> MSEYMDDVDREFINCLFPSYLLQQPVAYDLWILYLQHRKLFHKLKNTNLINADENPTGVGMGRTKLTALTRKEIWSKLMNLGVLGTISFEAVNDDYLIQVYKYFYPDVNDFTLRFGVKDSNKNSVRVMKASSDMRKNAQELLEPVLSEREMALNSNTSLENDRNDDDDDDDDDDDDDDDDDDDDDESDLESLEGEVDTDTDDNNEGDGSDNHEEGGEEGSRGADADVSSAQQRAERVADPWIYQRSRSAINIETESRNLWDTSDKNSGLQYYPPDQSPSSSFSSPRVSSGNDKNDNEATNVLSNSGSKKKNSMIPDIYKILGYFLPSRWQAQPNNSLQLSQDGITHLQPNPDYHSYMTYERSSASSASTRNRLRTSFENSGKVDFAVTWANKSLPDNKLTIFYYEIKVLSVTSTESAENSNIVIGYKLVENELMEATTKKSVSRSSVAGSSSSLGGSNNMSSNRVPSTSFTMEGTQRRDYIYEGGVSAMSLNVDGSINKCQKYGFDLNVFGYCGFDGLITNSTEQSKEYAKPFGRDDVIGCGINFIDGSIFFTKNGIHLGNAFTDLNDLEFVPYVALRPGNSIKTNFGLNEDFVFDIIGYQDKWKSLAYEHICRGRQMDVSIEEFDSDESEEDETENGPEENKSTNVNEDLMDIDQEDGAAGNKDTKKLNDEKDNNLKFLLGEDNRFIDGKLVRPDVNNINNLSVDDGSLPNTLNVMINDYLIHEGLVDVAKGFLKDLQKDAVNVNGQHSESKDVIRHNERQIMKEERMVKIRQELRYLINKGQISKCINYIDNEIPDLLKNNLELVFELKLANYLVMIKKSSSKDDDEIENLILKGQELSNEFIYDTKIPQSLRDRFSGQLSNVSALLAYSNPLVEAPKEISGYLSDEYLQERLFQVSNNTILTFLHKDSECALENVISNTRAMLSTLLEYNAFGSTNSSDPRYYKAINFDEDVLNLXXXXXXXXXXXXXXXXXXXXXXXXXXXXXXXXXXXXXXXXXXXXXXXXXXXXXXXXXXXXXXXXXXXXXXXX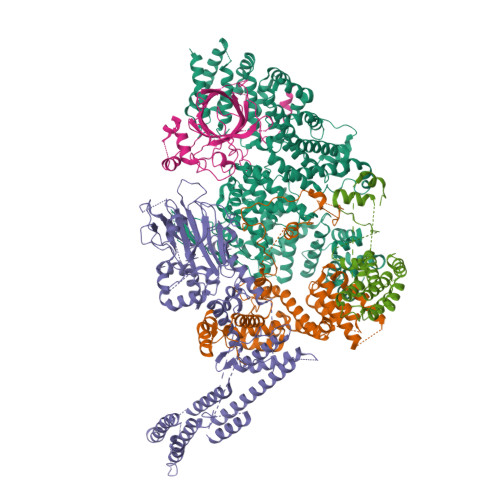XXXXXXXXXXXXXXXXXXXXXXXXXXXXXXXXXX;> MINNPKVDSVAEKPKAVTSKQSEQAASPEPTPAPPVSRNQYPITFNLTSTAPFHLHDRHRYLQEQDLYKCASRDSLSSLQQLAHTPNGSTRKKYIVEDQSPYSSENPVIVTSSYNHTVCTNYLRPRMQFTGYQISGYKRYQVTVNLKTVDLPKKDCTSLSPHLSGFLSIRGLTNQHPEISTYFEAYAVNHKELGFLSSSWKDEPVLNEFKATDQTDLEHWINFPSFRQLFLMSQKNGLNSTDDNGTTNAAKKLPPQQLPTTPSADAGNISRIFSQEKQFDNYLNERFIFMKWKEKFLVPDALLMEGVDGASYDGFYYIVHDQVTGNIQGFYYHQDAEKFQQLELVPSLKNKVESSDCSFEFA;> MTVAYSLENLKKISNSLVGDQLAKVDYFLAPKCQIFQCLLSIEQSDGVELKNAKLDLLYTLLHLEPQQRDIVGTYYFDIVSAIYKSMSLASSFTKNNSSTNYKYIKLLNLCAGVYPNCGFPDLQYLQNGFIQLVNHKFLRSKCKIDEVVTIIELLKLFLLVDEKNCSDFNKSKFMEEEREVTETSHYQDFKMAESLEHIIVKISSKYLDQISLKYIVRLKVSRPASPSSVKNDPFDNKGVDCTRAIPKKINISNMYDSSLLSLALLLYLRYHYMIPGDRKLRNDATFKMFVLGLLKSNDVNIRCVALKFLLQPYFTEDKKWEDTRTLEKILPYLVKSFNYDPLPWWFDPFDMLDSLIVLYNEITPMNNPVLTTLAHTNVIFCILSRFAQCLSLPQHNEATLKTTTKFIKICASFAASDEKYRLLLLNDTLLLNHLEYGLESHITLIQDFISLKDEIKETTTESHSMCLPPIYDHDFVAAWLLLLKSFSRSVSALRTTLKRNKIAQLLLQILSKTYTLTKECYFAGQDFMKPEIMIMGITLGSICNFVVEFSNLQSFMLRNGIIDIIEKMLTDPLFNSKKAWDDNEDERRIALQGIPVHEVKANSLWVLRHLMYNCQNEEKFQLLAKIPMNLILDFINDPCWAVQAQCFQLLRNLTCNSRKIVNILLEKFKDVEYKIDPQTGNKISIGSTYLFEFLAKKMRLLNPLDTQQKKAMEGILYIIVNLAAVNENKKQLVIEQDEILNIMSEILVETTTDSSSYGNDSNLKLACLWVLNNLLWNSSVSHYTQYAIENGLEPGHSPSDSENPQSTVTIGYNESVAGGYSRGKYYDEPDGDDSSSNANDDEDDDNDEGDDEGDEFVRTPAAKGSTSNVQVTRATVERCRKLVEVGLYDLVRKNITDESLSVREKARTLLYHMDLLLKVK;> MTISTLSNETTKSGSCSGQGKNGGKDFTYGKKCFTKEEWKEQVAKYSAMGELYANKTIHYPLKIQPNSSGGSQDEGFATIQTTPIEPTLPRLLLNYFVSMAYEDSSIRMAKELGFIRNNKDIAVFNDLYKIKERFHIKHLIKLGRINEAMEEINSIFGLEVLEETFNATGSYTGRTDRQQQQQQQQFDIDGDLHFKLLLLNLIEMIRSHHQQENITKDSNDFILNLIQYSQNKLAIKASSSVKKMQELELAMTLLLFPLSDSADSGSIKLPKSLQNLYSISLRSKIADLVNEKLLKFIHPRIQFEISNNNSKFPDLLNSDKKIITQNFTVYNNNLVNGSNGTKITHISSDQPINEKMSSNEVTAAANSVWLNQRDGNVGTGSAATTFHNLENKNYWNQTSELLSSSNGKEKGLEFNNYYSSEFPYEPRLTQIMKLWCWCENQLHHNQIGVPRVEN;> MAEKSIFNEPDVDFHLKLNQQLFHIPYELLSKRIKHTQAVINKETKSLHEHTAALNQIFEHNDVEHDELALAKITEMIRKVDHIERFLNTQIKSYCQILNRIKKRLEFFHELKDIKSQNSGTSHNGNNEGTRTKLIQWYQSYTNILIGDYLTRNNPIKYNSETKDHWNSGVVFLKQSQLDDLIDYDVLLEANRISTSLLHERNLLPLISWINENKKTLTKKSSILEFQARLQEYIELLKVDNYTDAIVCFQRFLLPFVKSNFTDLKLASGLLIFIKYCNDQKPTSSTSSGFDTEEIKSQSLPMKKDRIFQHFFHKSLPRITSKPAVNTTDYDKSSLINLQSGDFERYLNLLDDQRWSVLNDLFLSDFYSMYGISQNDPLLIYLSLGISSLKTRDCLHPSDDENGNQETETATTAEKEVEDLQLFTLHSLKRXXXXXXXXXXXXXXXXXXXXXXXXXXXXXXXXXXXXXXXXXXXXXXXX> MIYKTSKEIQKSDQRIIQQRVENSIINNQIYQKSLKRKTSKRKVRHQANKKNFQKEMSEVEDTLNRIKTHKTVLGYLIVNSEGGVVRGAFKDEEESKNIANSIPLLTKKARSVVRDLDPTNDLVFLRIQTKLNEIMVAPDDEFSLIVIQTKGEK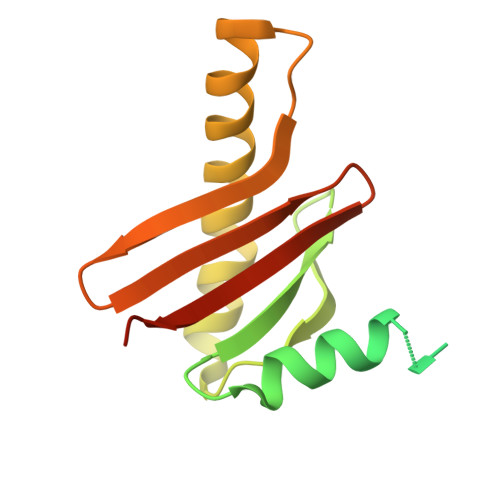RDEND> HHHHHHSSGLVPRGSHMTDIRSETAELRAELVERVHKFGPVFADGVAEGERERRLPDATVRAIDQSQLAMLWTAKSYGGLETDVRTMSEVAKVLSHYCPSTSWVVNNVNGSNLLASKFPRAALDEVFGDAPGAKLASVFAAAGTAVRTPGGYRLTGSWPYGTGILHDDWAILVAREVDADGEPVGGLSMLVPARDLTVEDTWHTVGMRATGSHTVVLRDTFVPEHRVISGELQRSRESATDLGLPPLFRTAAIAAMAVVCASVVLGAGQAARALVVEKAPTRGIAPSKYTRQTDSRTFVSSLGRTALSIDAAEMHVARAATALDDAAYDAVALPDSELLRIRGDVGQAVSLVTTALDELLWAHGAASFAESNPLQRYWRDANTAARHAMLNVHVGHELYGGSFFGLDPIVPSL

In vitro characterization, bioinformatics and structural investigations revealed that XiaF is a new member of the group D FMOs, monooxygenases that receive reduced FAD/FMN from a NAD(P)H-dependent flavin reductase and assemble in a tetrameric ACAD-fold composed of N- and C-terminal helical domains and a central β-sheet domain35. At the heart of the biosynthetic pathway, however, we discovered an unusual cyclization cascade involving the non-canonical terpenoid cyclases XiaE and XiaF22. Here we report the in vitro reconstitution of XiaF and a designated flavoenzyme-reductase, which jointly mediate a cryptic indole hydroxylation step that has been proposed to be a key step in non-canonical terpenoid cyclization. Accordingly, in the terpenoid pathway C-3 hydroxylation of the indole ring of indosespene by C4a-hydroperoxyflavin as the electrophilic oxygenating species yields a reactive intermediate (most likely the 3-hydroxyiminium cation 9, although deprotonation to yield an hydroxyindolenine intermediate is also conceivable) that is prone to nucleophilic attack of the exo-methylene group, resulting in the pentacyclic intermediate 16.

To further characterize the non-canonical terpenoid cyclase and the cryptic hydroxylation reaction, we carried out protein crystallization and modelling experiments. The intermolecular interactions between the individual subunits are solely formed between the C-terminal domains, whereas the N-terminal as well as the central β-sheet domains are directed towards the corners of the tetrahedron. The N-domain spans from Met1-Lys118, the β-sheet from Leu119-Ser213 and the C domain from Gly214-Leu397, which describes the typical architecture of a member of the ACAD superfamily. Cocrystallizations of XiaF with flavin proved to be challenging; initially no FAD bound to crystals could be observed when the oxidized cofactor was used. A similar result has been reported for FMN and the XiaF homologue C2-HpaH (4-hydroxyphenylacetate 3-hydroxylase), which has been shown to bind reduced FMN considerably better than oxidized FMN48.>MERLKLKEINVVNEITKILTGDYTFEESLKEVLKVLYSYLGVEHSFIAIREGNTLRIASSYGYFLNKDVAFKKGEGITGKVFQRGIPLVIPNVKHNSAFANKTGIGRLLTEKHALIAAPIKVGGEVKGVITIFKEFSDKESLENFYQTINVIGNLLGMFFKLREKFES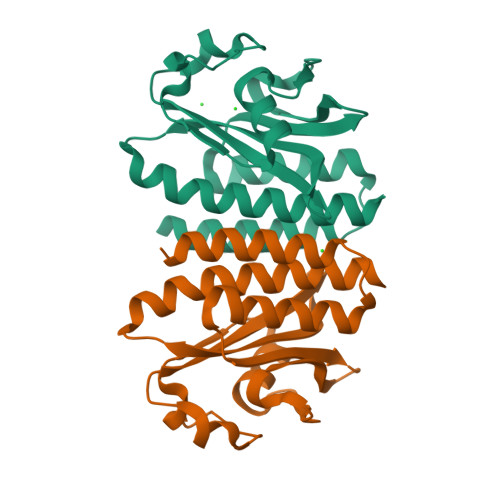EKKA[2x]ATP synthases convert energy of H+ electrochemical gradient across the membrane into energy of chemical bonds in ATP molecules by coupling of H+ transfer and ATP synthesis. All ATP synthases consist of two main parts, FO and F1. The most advanced are the studies of the c-ring which is a key part of the rotor. The proton flow passing between the ring and a-subunit2,8 drives rotation of the c-ring.

We present the first high-resolution structure of the c14-ring of cF1FO from spinach solved to 2.3 Å resolution. The space group of the crystals was determined to be I121, with the cell lattice parameters of a = 93.14 Å, b = 96.34 Å, с = 158.68 Å, α = γ = 90° and β = 106.72°. The c14-ring asymmetric unit cell contains one ring with 14 c-subunits in each. It shows a network of hydrogen bonds between water molecules and amino acids showing intersubunit contacts that determine the angle between c1 subunits and therefore the number of subunits in the c-ring. Glu61 side chain is directly hydrogen bonded to the Tyr66’ side chain and to the oxygen of Phe59 of the neighbor c-subunit. In opposite, interactions of inner helices create an extended hydrogen bonding network in the region close to the stroma inside the c14-ring, where double conformations of Gln34 side chains of neighbor subunits are connected both directly and via water molecule Wat203. Thr30 side chain and Val26 oxygen are hydrogen bonded via water molecule Wat202, additionally stabilizing the region. Ser21 side chain is bonded to the backbone of neighbor c-subunit via water molecule Wat201. The additional electron densities form three circles parallel to membrane plane at different levels with the distance of about 5.4 Å between each circle, which corresponds to the average distance between the bulky hydrophobic amino acids of the internal α-helix of the c-subunit. We hypothesize that the densities originate from isoprenoid molecules (presumably quinone isoprenoids, such as coenzyme Q in mitochondria, plastoquinone in chloroplasts and menaquinone in bacteria).

>MNPLIAAASVIAAGLAVGLASIGPGVGQGTAAGQAVEGIARQPEAEGKIRGTLLLSLAFMEALTIYGLVVALALLFANPFV[14x]> ASKSKVDNQFYSVEVGDSTFTVLKRYQNLKPIGSGAQGIVCAAYDAVLDRNVAIKKLSRPFQNQTHAKRAYRELVLMKCVNHKNIISLLNVFTPQKTLEEFQDVYLVMELMDANLCQVIQMELDHERMSYLLYQMLCGIKHLHSAGIIHRDLKPSNIVVKSDCTLKILDFGLARTAGTSFMMTPYVVTRYYRAPEVILGMGYKENVDIWSVGCIMGEMVRHKILFPGRDYIDQWNKVIEQLGTPCPEFMKKLQPTVRNYVENRPKYAG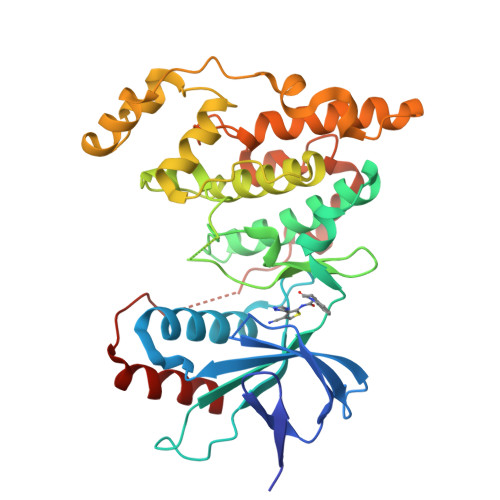LTFPKLFPDSLFPADSEHNKLKASQARDLLSKMLVIDPAKRISVDDALQHPYINVWYDPAEVEAPPPQIYDKQLDEREHTIEEWKELIYKEVMNS>[2x]AHDLEADVTMTGSDLVSCSYRSLAAPDLTLRDLLDIVETSQAHNARAQLTGALFYSQGVFFQWLEGRPAAVAEVMTHIQRDRRHSNVEILAEEPIAKRRFAGWHMQLSCSEADMRSLGLAESRQIVTVGR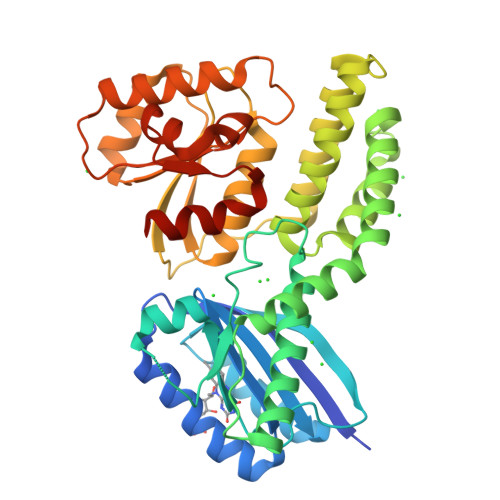SLVADNTNIFSFDRIAAVRRFLSDVCAARTLAPDTPVEADTFALYALTEAQAGRSGRAKAVARLSDLLSTDPLGRLTEVEELLRAHAPTAADFARLFEACAERLTRALAEDRISRMQVTLAYSALQMALRRIHHLPDPQKSVGAVLVAGVPGHKPILEAALAAEMLRAVGWSTSVVHPESVAALAARLKTSRTSTLVVAPSLLEGTEQEADTLRFVSALRARTDLPGLSILVGGRLAQLPPSKLKDSGADAGFAHLALLPAALARVASSAHHHHHH>[2x]GGMGQTLLDALNVRVVGSGERVLVLAHGFGTDQSAWNRILPFFLRDYRVVLYDLVCAGSVNPDFFDFRRYTTLDPYVDDLLHILDALGIDQCAYVGHSVSAMIGILASIRRPELFSKLILIGA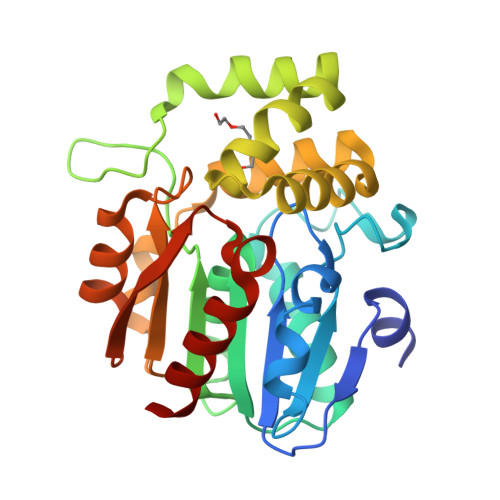SPRFLNDEDYHGGFEQGEIEKVFSAMEANYEAWVNGFAPLAVGAAVPAAVREFSRTLFNMRPDITLFVSRTVFNSDMRGVLGLVKVPCHIFQTARDHSVPASVATYLKNHLGGKNTVHWLNIEGHLPHLSAPTLLAQELRRALSHR>[3x]MHHHHHHHHAMTNNQ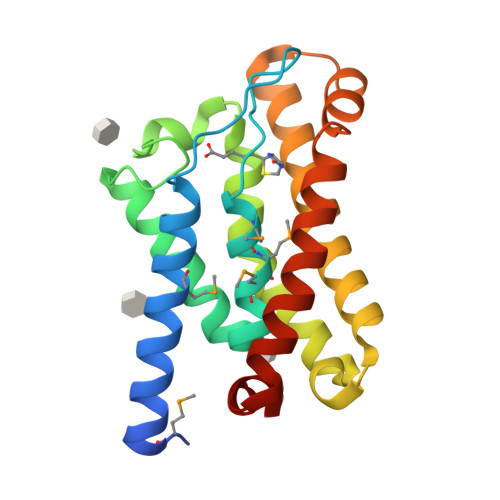KVKTLTYSAFMTAFIIILGFLPGIPIGFIPVPIILQNMGIMMAGGLLGPKYGTISVGAFLALALIGLPVLTGGNGGAASFLGPSGGYRIAWLFTPFLIGFFLKKLKITTSQNWFGELIIVLLFGVIFVDFVGAIWLSFQSNIPLLTSLISNLVFIPGDCIKAILTVVIVRRLRKQGGFELYFR>[2x]GSKRFYVKDHRNKAMINLH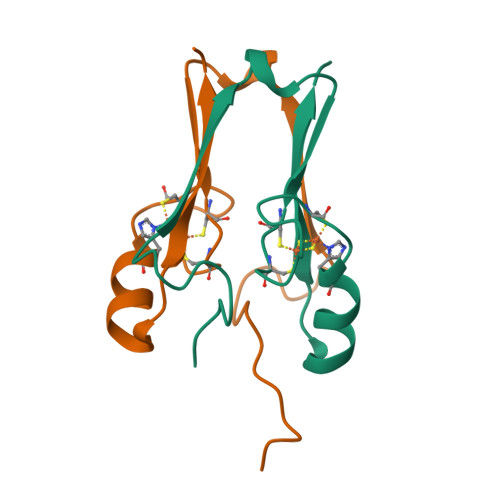IQKDNPKIVHAFDMEDLGDKAVYCRCWRSKKFPFCDGAHTKHNEETGDNVGPLIIKKKETAS> ANDTILPLNNIQGDILVGMKKQKERFVFFQVNDATSFKTALKTYVPERITSAAILISDPSQQPLAFVNLGFSNTGLQALGITDDLGDAQFPDGQFADAANLGDDLSQWVAPFTGTTIHGVFLIGSDQDDFLDQFTDDISSTFGSSITQVQALSGSARPGDQAGHEHFGFLNGISQPSVTGWETTVFPGQAVVPPGIILTGRDGDTGTRPSWALDGSFMAFRHFQQKVPEFNAYTLANAIPANSAGNLTQQEGAEFLGARMFGRWKSGAPIDLAPTADDPALGA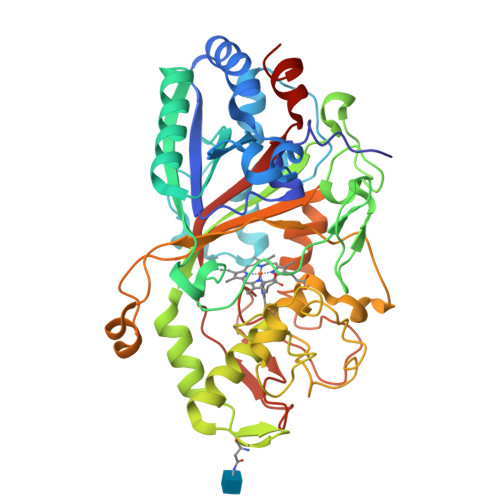DPQRNNNFDYSDTLTDETRCPFGAHVRKTNPRQDLGGPVDTFHAMRSSIPYGPETSDAELASGVTAQDRGLLFVEYQSIIGNGFRFQQINWANNANFPFSKPITPGIEPIIGQTTPRTVGGLDPLNQNETFTVPLFVIPKGGEYFFLPSISALTATIAA(2~{R})-4-[6-(2-fluoranyl-4-methoxy-phenyl)-3-oxidanylidene-1~{H}-pyrrolo[1,2-c]imidazol-2-yl]-2-methyl-2-methylsulfonyl-~{N}-oxidanyl-butanamide 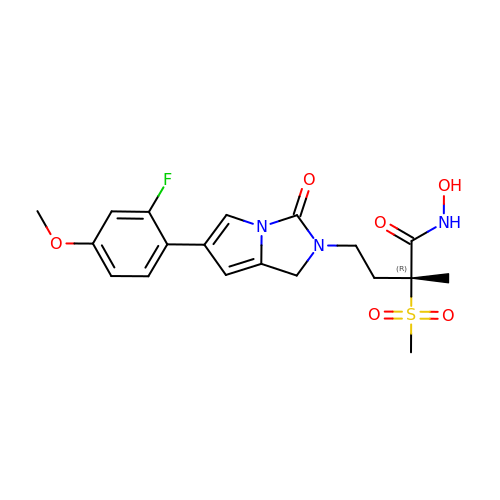| C19 H22 F N3 O6 S | ICRQKLIZNPTHKX-LJQANCHMSA-N>MEQRASLDSEESESPPQENSCLDPPDRDPNCKPPPVKPHIFTTRSRTRLFGKGDSEEASPLDCPYEEGGLASCPIITVSSVLTIQRPGDGPASVRPSSQDSVSAGEKPPRLYDRRSIFDAVAQSNCQELESLLPFLQRSKKRLTDSEFKDPETGKTCLLKAMLNLHNGQNDTIALLLDVARKTDSLKQFVNASYTDSYYKGQTALHIAIERRNMTLVTLLVENGADVQAAANGDFFKKTKGRPGFYFGELPLSLAACTNQLAIVKFLLQNSWQPADISARDSVGNTVLHALVEVADNTVDNTKFVTSMYNEILILGAKLHPTLKLEEITNRKGLTPLALAASSGKIGVLAYILQREIHEPECRHLSRKFTEWAYGPVHSSLYDLSCIDTCEKNSVLEVIAYSSSETPNRHDMLLVEPLNRLLQDKWDRFVKRIFYFNFFVYCLYMIIFTAAAYYRPVEGLPPYKLKNTVGDYFRVTGEILSVSGGVYFFFRGIQYFLQRRPSLKSLFVDSYSEILFFVQSLFMLVSVVLYFSQRKEYVASMVFSLAMGWTNMLYYTRGFQQMGIYAVMIEKMILRDLCRFMFVYLVFLFGFSTAVVTLIEDGKYNSLYSTCLELFKFTIGMGDLEFTENYDFKAVFIILLLAYVILTYILLLNMLIALMGETVNKIAQESKNIWKLQRAITILDTEKSFLKCMRKAFRSGKLLQVGFTPDGKDDYRWCFRVDEVNWTTWNTNVGIINEDPGNCEGVKRTLSFSLRSGRVSGRNWKNFALVPLLRDASTRDRHATQQEEVQLKHYTGSLKPEDAEVFKDSMVPGEK[4x]

The capsaicin- and heat-activated receptor, TRPV1, has served as a model for deciphering lipid modulation, which is relevant to understanding how pro-algesic agents enhance channel activity in the setting of inflammatory pain. Identification of a pocket within the TRPV1 transmembrane core has provided initial clues as to how phosphoinositide lipids bind to and regulate the channel. Here we show that this regulatory pocket in rat TRPV1 can accommodate diverse lipid species, including the inflammatory lipid lysophosphatidic acid, whose actions are determined by their specific modes of binding. We captured several states of TRPV1 ranging from channels in which the VBP is empty to those bearing different bioactive lipids, including distinct phosphoinositide species, brominated phosphoinositide analogs and a pro-algesic lipid, lysophosphatidic acid (LPA). Together, our data show how the VBP accommodates a range of bioactive lipids and how occupancy of the site corresponds to the structural status of the pore.

To visualize the lipid–channel complex, we added LPA to nanodisc-reconstituted TRPV1 and determined a consensus cryo-EM map to a resolution of 3.0 Å. Through symmetry expansion and focused classification, we captured LPA bound within the vanilloid pocket in multiple stoichiometries, ranging from apo to all four subunits occupied. LPA displaces the endogenous PI lipid by occupying the upper region of the pocket that binds aliphatic tails. As in the case of vanilloid agonists, Y511 flips toward the VBP so that its hydroxyl group forms an H-bond with the ester carbonyl of the LPA tail. Moreover, S512, T550 and Y554 engage in H-bond interactions with the phosphate moiety of LPA, while the free hydroxyl of the glycerol backbone interacts with N551. Therefore, the RTX headgroup may be better suited for priming this salt bridge interaction as compared to LPA, which may help to explain the greater efficacy of RTX as an agonist. Together, these structures demonstrate that LPA utilizes similar molecular interactions as vanilloid agonists, such as RTX or capsaicin, for binding to TRPV1 and initiating gating. Reorientation of Y511 toward the VBP is a key step, allowing L574 on the S4–S5 linker to partially occupy the now vacant space, thereby facilitating movement of the S4–S5 linker toward the VBP. Movement of the S4–S5 linker enables the S5 and S6 helices to move away from the pore axis while providing space to accommodate a π–α helix transition in S6, which is associated with the loss of hydrophobic interactions between M682 and the S4–S5 linker. Our structures now show that LPA, an important inflammatory lipid, binds to the VBP and displaces the resident PI lipid, further validating this site as a key regulatory locus for the action of both endogenous and exogenous lipophilic agents.>[2x]ADPLLPYFDFDVPRNLTVTVGQTGFLHCRVERLGDKDVSWIRKRDLHILTAGGTTYTSDQRFQVLRPDGSANWTLQIKYPQPRDSGVYECQINTEPKMSLSYTFNVVEHHHHHH;>SRIVDPKFSSPIVNMTAPVGRDAFLTCVVQDLGPYKVAWLRVDTQTILTIQNHVITKNQRIGIANSEHKTWTMRIKDIKESDKGWYMCQINTDPMKSQMGYLDVVVHHHHHH[2x]

We have recently identified interactions between two groups of Drosophila IgSF (immunoglobulin superfamily) cell adhesion molecules with properties closely matching a neuronal chemoaffinity function: 21 Dpr proteins, named after the founding member Defective proboscis extension response, selectively bind nine proteins, now called the Dpr-interacting proteins, or DIPs. All 21 Dprs and nine DIPs are predicted to contain two and three immunoglobulin (IG) domains, respectively. Our previous work identified the first IG domains, termed IG1, as the domains mediating the Dpr–DIP interaction by the formation of a pseudo-symmetric IG1-IG1 heterocomplex using the GFCC’C’ face of the immunoglobulin fold. Therefore, Dprs and DIPs are strong candidates for a synapse specification or targeting function.

We chose complexes of Dpr1 and Dpr11, as they are reported to have neuronal phenotypes, and therefore these complex structures can be directly used to investigate the relationship between Dpr–DIP interactions and the observed phenotypes. We crystallized and solved the structures of Dpr1 IG1 with DIP-η IG1, and Dpr11 IG1 with DIP-γ IG1 +2. However, one method, the statistical coupling analysis (SCA) version 5, identified one pair of amino acids, Dpr His94 (Dpr1) and DIP Met132 (DIP-η). These two residues directly contact each other and cap the hydrophobic interior of the interface. With these data, we first investigated the His94 (Dpr1) to Glu126 (DIP-η) hydrogen bond, which appeared to be the only conserved side chain-to-side chain hydrogen bond among the three heterophilic complexes based on sequence conservation. For the Dpr1–DIP-η and Dpr6–DIP-α complexes, His-to-Ala mutation unexpectedly increased affinity despite removing a hydrogen bond and significant packing. Overall, it appears that Dpr–DIP specificity is encoded not only by relationships between pairs of Dpr and DIP residues (e.g., K144 in Dpr1 with T83 in DIP-η, Figure 3d1), but also through coupling of multiple residues, and through shape complementarity, where rotameric changes help create complementary surfaces. The main chain positions of a DIP-η bound to either another DIP-η or Dpr1 are virtually identical, and surprisingly, most side chains also preserve their rotameric states. We believe that interdomain flexibility and long low-complexity ‘stalk’ regions linking the IG domains to the membrane would enable cis dimerization for homodimeric DIPs, such as DIP-α and DIP-η. In fact, our SPR experiments where DIP-η is captured on solid support at high densities reports much higher apparent KD values for the Dpr1–DIP-η interaction (23 µM vs 4.0 µM measured when non-dimerizing Dpr1 is captured on SPR chip; Figure 4—figure supplements 1,3), as the cis DIP-η homodimer formation on the chip likely competes with Dpr1 binding.> SKVALITGITGQDGSYLAEFLLEKGYMVYGIIRRSSSFNTGRVEHLYKDIHITKAKFKLLYGDLTDTGNLISIIAKIKPDEIYNLAAQSHVKVSFEMPEYTANVDGIGTLRLLEAIRACGLEKKTKFYQASTSELYGLVQEVPQKETTPFYPRSPYACAKLYSYWIVVNYREAYNMFALNGILFNHESIRRGPTFVTRKITMAVARIKLGLQDCLYLGNLDAERDWGHAKDYVEAMWLMLQQEQPRDFCVATGEKHSVREFVEKAFACIGQTV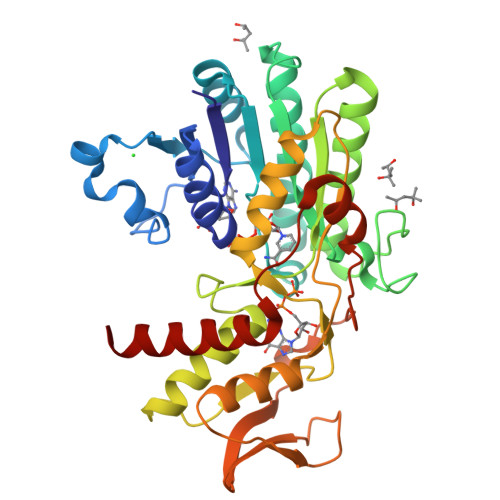EWKGERGTVEEHGVVDGVVRVRVDPRYFRPTEVDQLLGDPTLAETVLGWKRKVSFEELVRGMVEGDIELLQS4-azanyl-2-[(3~{S})-2,5-bis(oxidanylidene)pyrrolidin-3-yl]isoindole-1,3-dione | C12 H9 N3 O4 | 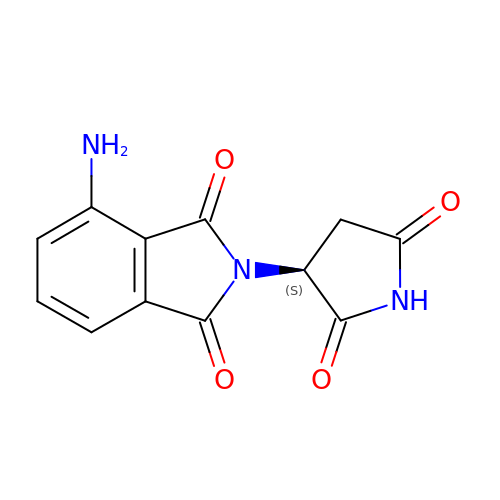MSHTVRYXGFREAN-ZETCQYMHSA-N>MERKQKNSLFNYIYSLMDVRGKFLFFSMLFITSLSSIIISISPLILAKITDLLSGSLSNFSYEYLVLLACLYMFCVISNKASVFLFMILQSSLRINMQKKMSLKYLRELYNENITNLSKNNAGYTTQSLNQASNDIYILVRNVSQNILSPVIQLISTIVVVLSTKDWFSAGVFFLYILVFVIFNTRLTGSLASLRKHSMDITLNSYSLLSDTVDNMIAAKKNNALRLISERYEDALTQENNAQKKYWLLSSKVLLLNSLLAVILFGSVFIYNILGVLNGVVSIGHFIMITSYIILLSTPVENIGALLSEIRQSMSSLAGFIQRHAENKATSPSIPFLNMERKLNLSIRELSFSYSDDKKILNSVSLDLFTGKMYSLTGPSGSGKSTLVKIISGYYKNYFGDIYLNDISLRNISDEDLNDAIYYLTQDDYIFMDTLRFNLRLANYDASENEIFKVLKLANLSVVNNEPVSLDTHLINRGNNYSGGQKQRISLARLFLRKPAIIIIDEATSALDYINESEILSSIRTHFPDALIINISHRINLLECSDCVYVLNEGNIVASGHFRDLMVSNEYISGLASVTE[2x]

The ABC transporter McjD exports the antibacterial peptide MccJ25 in Escherichia coli. Four genes are required for the biosynthesis and export of MccJ25 (Duquesne et al, 2007b): mcjA encodes the linear precursor of MccJ25; mcjB and mcjC encode enzymes involved in the post‐translational modification of McjA to the lasso structure; and mcjD encodes an ABC exporter that is required for both MccJ25 secretion and self‐immunity of the producing strain towards MccJ25 (Choudhury et al, 2014). We have previously functionally characterized and determined the high‐resolution structure of McjD from Escherichia coli (Choudhury et al, 2014). Its core architecture is composed of a dimeric transmembrane domain (TMD) of 12 transmembrane (TM) helices, which forms the translocation pathway across the membrane bilayer and contains the ligand binding site, and a dimeric nucleotide binding domain (NBD) where ATP binds and is hydrolysed. In this study, we have determined its structure in a novel conformation, apo inward‐occluded and a new nucleotide‐bound state, high‐energy outward‐occluded intermediate state, with a defined ligand binding cavity.

In order to gain a detailed understanding of the conformations that McjD adopts during the transport cycle, we have determined its structure in the presence of the transition state analogue ADP‐VO4 (mimic of ATP hydrolysis) and in the absence of nucleotides, that is in the apo form, at 3.4 Å and 4.7 Å resolution, respectively. Clear electron density was observed for ADP‐VO4 and Mg2+ (Fig EV1A–D). The presence of vanadate was verified by collecting the data close to the vanadium K‐edge, 2.26 Å wavelength and calculating anomalous difference electron density maps (Fig EV1C). At both NBDs, two strong electron density peaks of 14 and 20 sigma, respectively, confirmed the presence of two VO4 groups. McjD‐ADP‐VO4 is almost identical to the McjD‐AMPPNP, as the two structures can be superimposed with a root‐mean‐square deviation (rmsd) of 0.7 Å over 560 Cα atoms (Fig EV2A and B). In contrast to the MsbA‐ADP‐VO4 structure that adopts an outward‐open conformation as a result of domain intertwining (Ward et al, 2007), the McjD‐ADP‐VO4 structure is outward‐occluded without domain intertwining. We call it here high‐energy intermediate outward‐occluded. The TMD dimer interface in McjD‐ADP‐VO4 is formed between TM2 and TM5/TM6 from one subunit with the equivalent TMs from the opposite subunit similar to the McjD‐AMPPNP structure. In the presence of ADP‐VO4, the NBDs are dimerized with the P‐loop and ABC signature motifs involved in the binding of the nucleotide. The McjD‐ADP‐VO4 structure represents the transition state of a water molecule making a nucleophilic attack on the γ‐phosphate of ATP.>GPGSMSLRGKTMFISGGSRGIGLAIAKRVAADGANVALVAKSAEPHPKLPGTIYTAAKEIEEAGGQALPIVGDIRDGDAVAAAVAKTVEQFGGIDICVNNASAINLGSIEE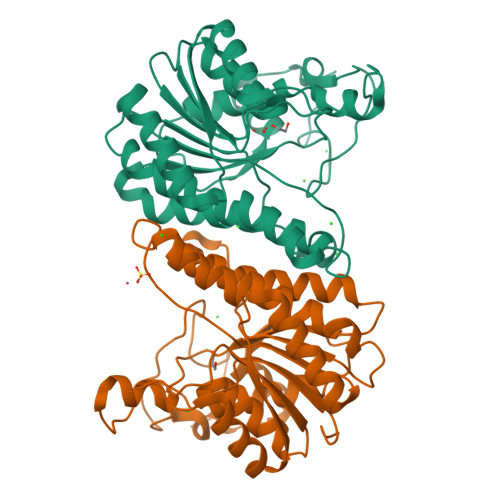VPLKRFDLMNGIQVRGTYAVSQSCIPHMKGRDNPHILTLSPPIRLEPKWLRPTPYMMAKYGMTLCALGIAEELRDAGIASNTLWPRTTVATAAVQNLLGGDEAMARSRKPEVYADAAYVVLNKPSSYTGNTLLCEDVLLESGVTDLSVYDCVPGSELGVDLWVDSPNPPGYTGP[2x]>SNAMKLLNTLVCIIGLTSFSSSAKLVNAEHLDALYQKVTVANKTELGLIHIYSEFPDYRWVKDPIEGVSAIDDVARAAIFYQRQYQATGSAADLEKVKSLVEFILYQRADNGYFYNFIYPDHSINKEYKTSVAEPNWWTWRALWALTQVYPTLVKTDNALAQRTRETIFATIDVIYKDFNFKQTRGEKEGVAVPEWLPHTAGDQASVLLMALSDAQALEAKPEIEKMMRSLAAGIMLMQVKDTSSPVNGAFLSWQNLWHGYGNSQAYALLVAGNRLGDRDMIKAAFNELDHFHPWLISNGLLNEFTVRQQGEKVTL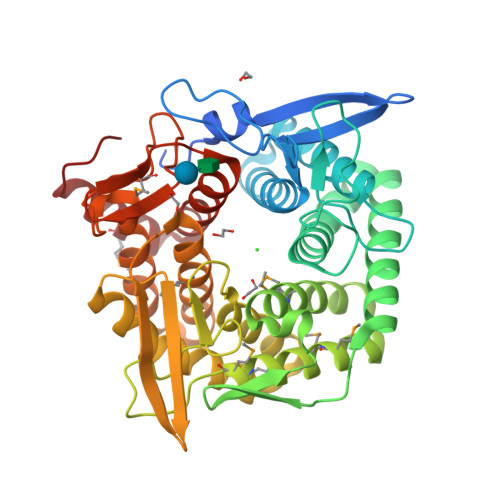IEQKKFSQIAYIIRPMVFANIKAWEISRDAVYLERAVDLSLWFFKNNPAQAQMYYPVTGIAFDGIDSATTVNKNSGAESTIEALLTLQLIESIPDAKRMLESALEKRNIKQ[2x]>MGSTPTDTTQNPQINWTKGGQAQSSSLNGQVFQVAVGSNFNPLNFTNSNGENIIVSAQQSKNNTTFASIEATSNPVNTSEAGRYYNVTLTATGNTGKKTTATYTVLITSSQKQTLYGNGESTISTYSIYGNNVLSNSTTFKDGDQVYVSDQTKTVGGVSYSQVSPKSKNDANSSNIWVKTSLE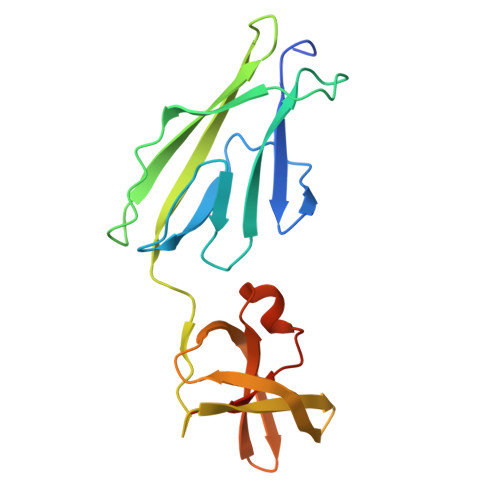HHHHHH[6x]> EDND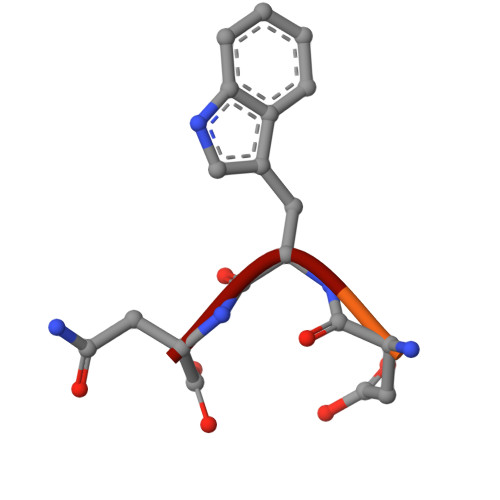WN> MNLFRKKPIQLLMKESGAKGASLRKELGAFDLTMLGIGAIIGTGIFVLTGVAAAEHAGPALVLSFILSGLACVFAALCYAEFASTVPVSGSAYTYSYATFGELIAWILGWDLILEYGVASSAVAVGWSGYFQGLLSGFGIELPKALTSAYDPAKGTFIDLPAIIIVLFITFLLNLGAKKSARFNAVIVAIKVAVVLLFLAVGVWYVKPENWTPFMPYGFSGVATGAATVFFAYIGFDAVSTAAEEVRNPQRDMPIGIIVSLLVCTLLYIAVSLVLTGIVPYEQLNVKNPVAFALNYIHQDWVAGFISLGAIAGITTVLLVSMYGQTRLFYAISRDGLLPKVFARISPTRQVPYVNTWLTGAAVAVFAGIIPLNKL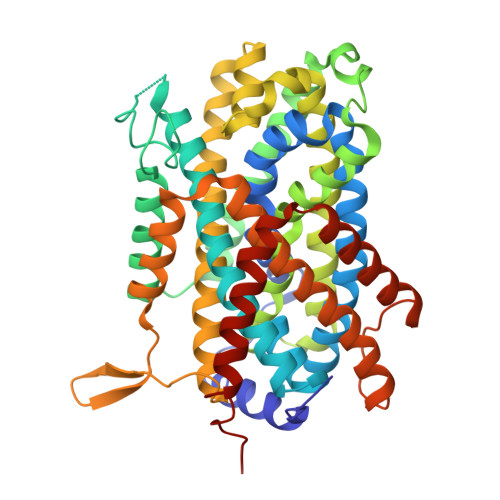AELTNIGTLFAFITVSIGVLVLRKTQPDLKRAFRVPFVPVVPILAVLFCGYLVLQLPAMTWIGFVSWLLIGLVIYFIYGRKHSELN(2R,5R)-2-[(2S,3R)-3-hydroxy-1-oxobutan-2-yl]-5-[(2R)-tetrahydrofuran-2-yl]-2,5-dihydro-1,3-thiazole-4-carboxylic acid | C12 H17 N O5 S | 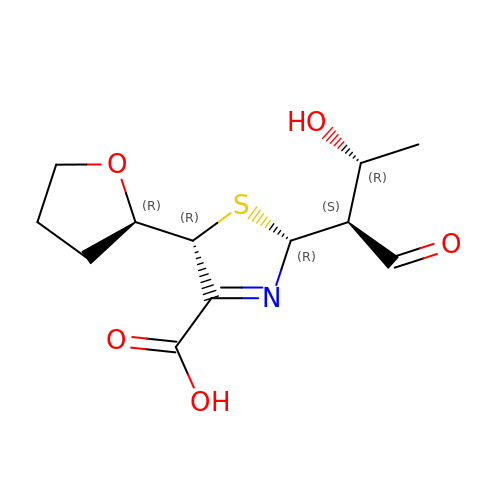FHQOUTNMKXYVEY-MKSGQPMJSA-N> MDEELENEETKKKKGGSLVIIIVILLFVLLLSIMGVIAWLISSSSSDESEVKEAPKEEAKADKPKVSAPTQRGSDFA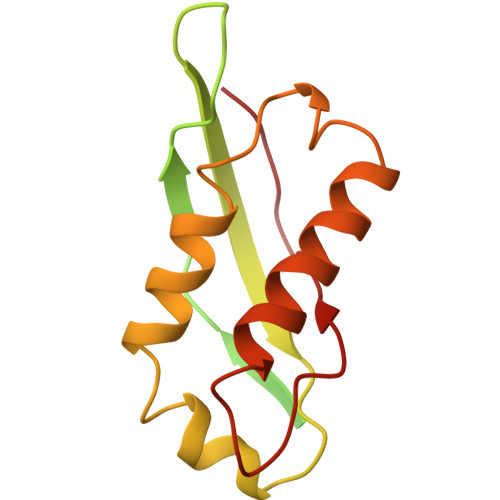NIGPMYPLDPFTLNLLSDSGSRYVKCTIELEQNSELLKPELDKKVPVIRDIIIRTLTAKTFEEVSTQKGKERLKDELVGKINEILTDGFIKNVYFTDFVVS> QDGKTTFEKEGGGGRGPRILENMHESSCKYE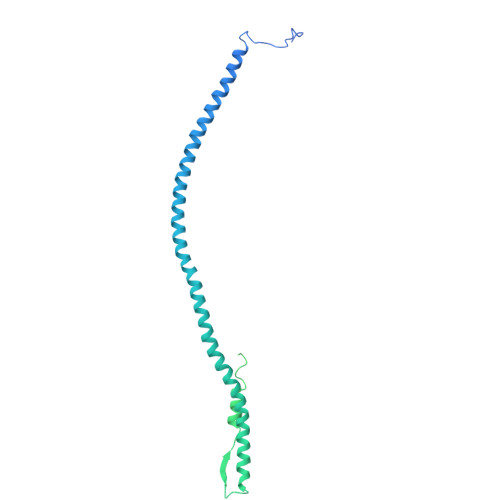KNWPICVDDDWGTKCPSCCRMQGIIDDTDQNYSQRIDNIRQQLADSQNKYKTSNRVIVETINILKPGLEGAQQLDENYGHVSTELRRRIVTLKQRVATQVNRIKALQNSIQEQVVEMKRLEVDIDIKIRACKGSCARSFDYQVDKEGYDNIQKHLTQASSIDMHPDFQTTTLSTLKMRPLKDSNVPEHFKLKPSPEMQAMSAFNNIKQMQVVLERPETDHVAEARGDSSPSHTGKLITSSHRRESPSLVDKTSSASSVHRCTRTVTKKVISGPDGPREEIVEKMVSSDGSDCSHLQGGREGSTYHFSGTGDFHKLDRLLPDLESFFTHDSVSTSSRHSIGSSTSSHVTGAGSSHLGTGGKDKFTDLGEEEEDDFGGLQPSGFAAGSASHSKTVLTSSSSSFNKGGSTFETKSLKTRETSEQLGGVQHDQSAEDTPDFKARSFRPAAMSTRRSYNGKGTQK> HM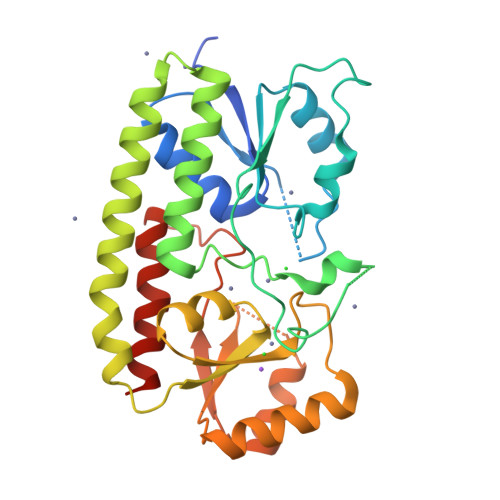GTGSLGGGFPGKGMKIVTSFYPIYAMVKEVSGDLNDVRMIQSSSGIASFEPSANDIAAIYDADVFVYHSHTLESWAGSLDPNLKKSKVKVLEASEGMTLERVPGLEDVEAGDGVDEKTLYDPHTWLDPEKAGEEAQIIADKLSEVDSEHKETYQKNAQAFIKKAQELTKKFQPKFEKATQKTFVTQHTAFSYLAKRFGLNQLGIAGISPEQEPSPRQLTEIQEFVKTYKVKTIFTESNASSKVAETLVKSTGVGLKTLNPLESDPQNDKTYLENLEENMSILAEELKGNLYFQ>[2x]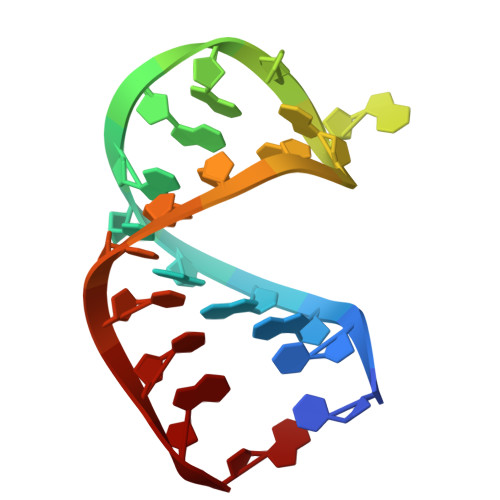CUGGGCGGGCGACCGCCUGG> GPMTFAVSVGGRRVDCEPGQTLLEAFLRGGVWMPNSCNQGTCGTCKLQVLSGEVDHGGAPEDTLSAEERASGLALACQARPLADTEVRSTADAGRVTHPLRDLTATVLEVADIARDTRRVLLGLAEPLAFEAGQYVELVVPGSGARRQYSLANTADEDKVLELHVRRVPGGVATDGWLFDGLAAGDRVEATGPLGDFHLPPPDEDDGGPMVLIGGGTGLAPLVGIARTALARHPSREVLLYHGVRGAADLYDLGRFAEIAEEHPGFRFVPVLSDEPDPAYRGGFPTDAFVEDVPSGRGWSGWLCGPPAMVEAGVKAFKRRRMSPRRIHREKFTP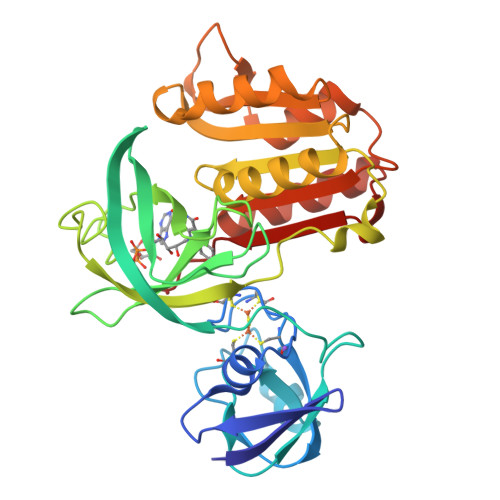AS3-[(5-acetyl-2-ethoxyphenyl)carbamoyl]benzoic 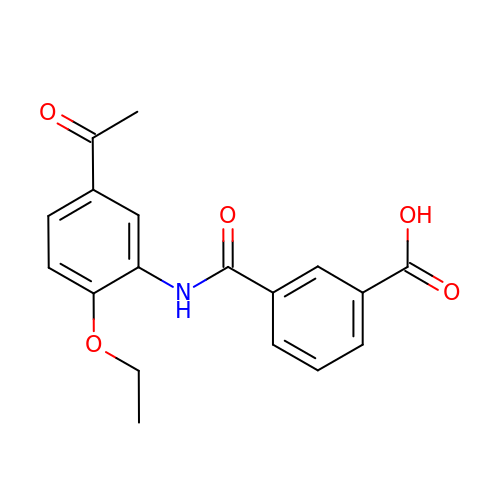acid | C18 H17 N O5 | GFOBMGVVDGTGAJ-UHFFFAOYSA-N>GGGHMLNTPFSPWPSFTQIEADAVSRVLLSNQVNYWTGQECRQFETEFAEWADSKYAIAMGNGTLALDVALQALDIGAGDEVIVTPRTFIASISSVVNIGATPVFSDVDEATGNITPESIAAVLTDKTKGIVCVHLAGWPCDMDGIMALADKHNLYVIEDCAQAHGATYKGRSVGSIGHIGAWSFCQDKIMTTGGEGGMVTTNDEQLWRKMWAYKDHGKSYAAVYETDHAPGYRWLHESFGTNWRMTEMQAVLGRIQLKRMPDWTAKRTANAQTILDACAKWEAKGYLSVPRLEESVQFADSTHAYYKLYVYVQSDNLPK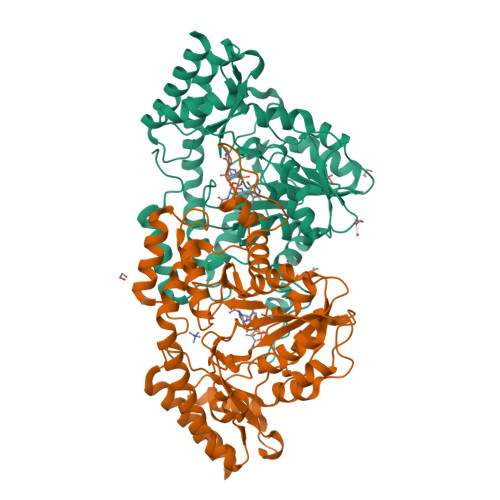EWSRDRIIREINDLGVPCFSGSASEVYLEKAFDNTGLRPENRLPVAKQLGETSLMFLVHPTLTEDEIKQTVQAIDGVFANIHNQ[2x]>AQVINTFDGVADYLQTYHKLPDNYITKSEAQALGWVASKGNLADVAPGKSIGGDIFSNREGKLPGKSGRTWREADINYTSGFRN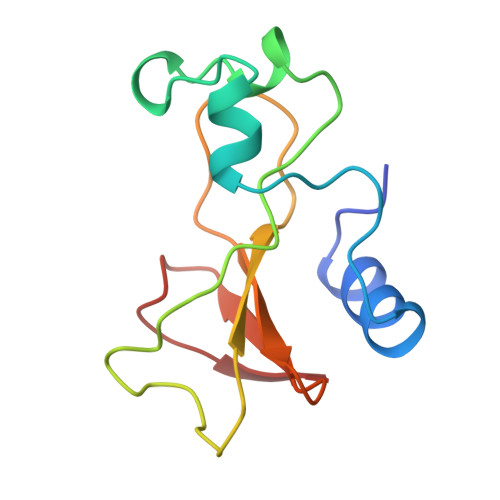SDRALYSSDWLIYKTTDHYQTFTKIR[3x]> VHFCDKCGLPIKVYGRMIPCKHVFCYDCAILHEKKGDKMCPGCSDPVQRIEQC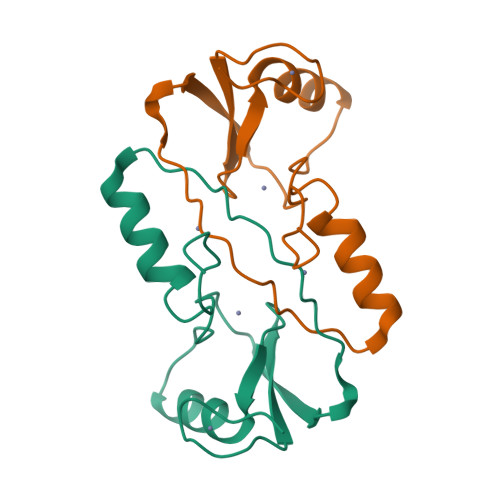TRGSLFMCSIVQGCKRTYLSQRDLQAHINHRHMRAGKPVTRASLENVH>SMTESTVDRINGITPSALDLIGNTPLIALDRLWPGPGRLLAKCEFLNPTASLKDRSSYYMIAKAKESGQLKDGESVIEVTSGNQGGGIACVTAVMGHPFTVTMSKGNSPQRAIMMNALGANVILVDQVTGKPGNVTADDVAAAEETAMKIREETNAYYVDQFNNPTNCLAHYETTGPEIWRQTNGRIDAFLVGCGTGGCFVGTSKFLKEKNPNVRCFVVEPEGCQPIAGCTITKPLHLLQGSGYGCVPTLFDKKVYNDSISVSDEEAIEYRKLLGQKEGLFCGFTTGGNIAAAIKLLKSGQLPKDAWVVTILCDSGLKYPE[2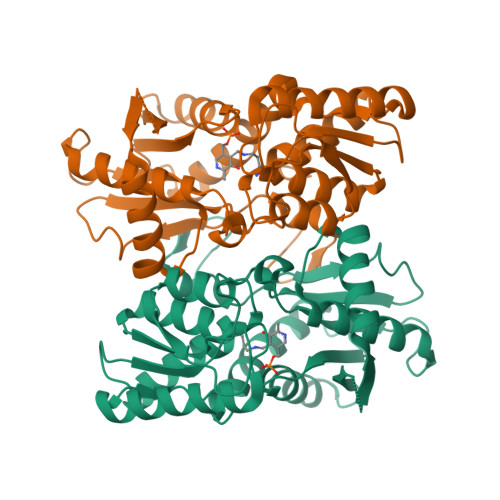x]>CELDRDPEGKDFQQPYTSFVQTKQNRDGLYALLRNTENPRMHFYQELQSDMYCTTITDGNSLAPFVNWDLGILNDHGRADEDEVSGIAGYYFVYNRLNQQANAFVNNTEAALQNQVYKNSTEIANAKSFLAEGKVLQALAIWRLMDRFSFHESVTEVNSGAKDLGVILLKEYNPGYIGPRATKAQCYDYILSRLSEAIEVLPENRESVLYVSRDYAYALRARIYLALGEYGKAAADAKMVVDKYPLIGAADASEFENIYRSDANNPEIIFRGFASATLGSFTATTLNGAAPAGKDIKYNPSAVPFQWVVDLYENEDFRKSVYIAKVVKKDKGYLVNKFLEDKAYRDVQDKPNLKVGARYFSVAEVYLILVESALQTGDTPTAEKYLKALSKARGAEVSVVNMEALQAERTRELIGEGSRLRDMVRWSIPNNHDAFETQPGLEGFANTTPLKAQAPVGFYAYTWEFPQRDRQTNPQLIKNWPIHHHHHH[4x];>QNRTVKGTVISSEDNEPLIGANVVVVGNTTIGAATDLDGNFTLSVPANAKMLRVSYSGMTTKEVAIANVMKIVLDPDSKVLEQVVVLGYGTGQKLSTVSGSVAKVSSEKLAEKPVANIMDALQGQVAGMQVMTTSGDPTAVASVEIHGTGSLGASSAPLYIVDGMQTSLDVVATMNPNDFESMSVLKDASATSIYGARAANGVVFIQTKKGKMSERGRITFNASYGISQILNTKPLDNMMTGDELLDFQVKAGFWGNNQTVQKVKDMILAGAEDLYGNYDSLKDEYGKTLFPVDFNHDADWLKALFKTAPTSQGDISFSGGSQGTSYYASIGYFDQEGMAREPANFKRYSGRLNFESRINEWLKVGANLSGAIANRRSADYFGKYYMGSGTFGVLTMPRYYNPFDVNGDLADVYYMYGATRPSMTEPYFAKMRPFSSESHQANVNGFAQITPIKGLTLKAQAGVDITNTRTSSKRMPNNPYDSTPLGERRERAYRDVSKSFTNTAEYKFSIDEKHDLTALMGHEYIEYEGDVIGASSKGFESDKLMLLSQGKTGNSLSLPEHRVAEYAYLSFFSRFNYGFDKWMYIDFSVRNDQSSRFGSNNRSAWFYSVGGMFDIYNKFIQESNWLSDLRLKMSYGTTGNSEIGNYNHQALVTV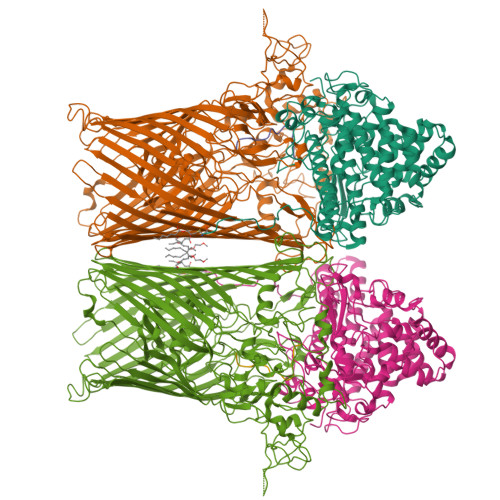NNYTEDAMGLSISTAGNPDLSWEKQSQFNFGLAAGAFNNRLSAEVDFYVRTTNDMLIDVPMPYISGFFSQYQNVGSMKNTGVDLSLKGTIYQNKDWNVYASANFNYNRQEITKLFFGLNKYMLPNTGTIWEIGYPNSFYMAEYAGIDKKTGKQLWYVPGQVDADGNKVTTSQYSADLETRIDKSVTPPITGGFSLGASWKGLSLDADFAYIVGKWMINNDRYFTENGGGLMQLNKDKMLLNAWTEDNKETDVPKLGQSPQFDTHLLENASFLRLKNLKLTYVLPNSLFAGQNVIGGARVYLMARNLLTVTKYKGFDPEAGGNVGKNQYPNSKQYVAGIQLSF[4x];>[2x]ASTTGGNSQRGGG;>[2x]ASTTGGNSQRGSG> QSMSVKGRIYSILKQIGSGGSSKVFQVLNEKKQIYAIKYVNLEEADNQTLDSYRNEIAYLNKLQQHSDKIIRLYDYEITDQYIYMVMECGNIDLNSWLKKKKSIDPWERKSYWKNMLEAVHTIHQHGIVHSDLKPANFLIVDGMLK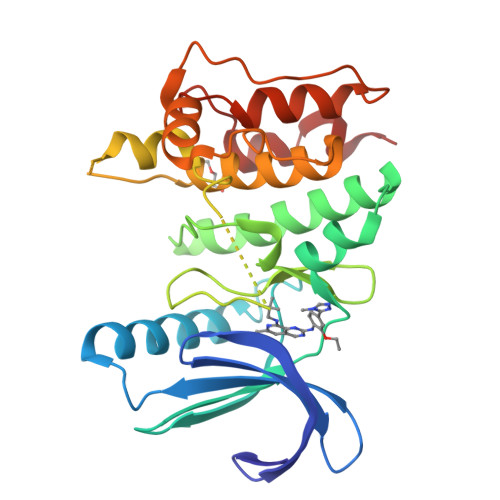LIDFGIANQMQPDTTSVVKDSQVGTVNYMPPEAIKDMSSSRENGKSKSKISPKSDVWSLGCILYYMTYGKTPFQQIINQISKLHAIIDPNHEIEFPDIPEKDLQDVLKCCLKRDPKQRISIPELLAHPYVQIQ>[8x]MAQILPIRFQEHLQLQNLGINPANIGFSTLTMESDKFICIREKVGEQAQVVIIDMNDPSNPIRRPISADSAIMNPASKVIALKAGKTLQIFNIEMKSKMKAHTMTDDVTFWKWISLNTVALVTDNAVYHWSMEGESQPVKMFDRHSSLAGCQIINYRTDAKQKWLLLTGISAQQNRVVGAMQLYSVDRKVSQPIEGHAASFAQFKMEGNAEESTLFCFAVRGQAGGKLHIIEVGTPPTGNQPFPKKAVDVFFPPEAQNDFPVAM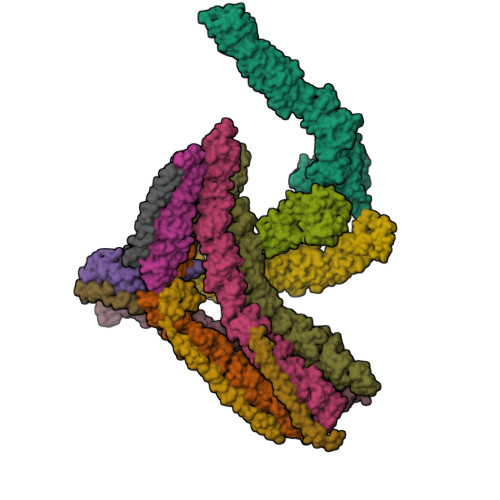QISEKHDVVFLITKYGYIHLYDLETGTCIYMNRISGETIFVTAPHEATAGIIGVNRKGQVLSVCVEEENIIPYITNVLQNPDLALRMAVRNNLAGAEELFARKFNALFAQGNYSEAAKVAANAPKGILRTPDTIRRFQSVPAQPGQTSPLLQYFGILLDQGQLNKYESLELCRPVLQQGRKQLLEKWLKEDKLECSEELGDLVKSVDPTLALSVYLRANVPNKVIQCFAETGQVQKIVLYAKKVGYTPDWIFLLRNVMRISPDQGQQFAQMLVQDEEPLADITQIVDVFMEYNLIQQCTAFLLDALKNNRPSEGPLQTRLLEMNLMHAPQVADAILGNQMFTHYDRAHIAQLCEKAGLLQRALEHFTDLYDIKRAVVHTHLLNPEWLVNYFGSLSVEDSLECLRAMLSANIRQNLQICVQVASKYHEQLSTQSLIELFESFKSFEGLFYFLGSIVNFSQDPDVHFKYIQAACKTGQIKEVERICRESNCYDPERVKNFLKEAKLTDQLPLIIVCDRFDFVHDLVLYLYRNNLQKYIEIYVQKVNPSRLPVVIGGLLDVDCSEDVIKNLILVVRGQFSTDELVAEVEKRNRLKLLLPWLEARIHEGCEEPATHNALAKIYIDSNNNPERFLRENPYYDSRVVGKYCEKRDPHLACVAYERGQCDLELINVCNENSLFKSLSRYLVRRKDPELWGSVLLESNPYRRPLIDQVVQTALSETQDPEEVSVTVKAFMTADLPNELIELLEKIVLDNSVFSEHRNLQNLLILTAIKADRTRVMEYINRLDNYDAPDIANIAISNELFEEAFAIFRKFDVNTSAVQVLIEHIGNLDRAYEFAERCNEPAVWSQLAKAQLQKGMVKEAIDSYIKADDPSSYMEVVQAANTSGNWEELVKYLQMARKKARESYVETELIFALAKTNRLAELEEFINGPNNAHIQQVGDRCYDEKMYDAAKLLYNNVSNFGRLASTLVHLGEYQAAVDGARKANSTRTWKEVCFACVDGKEFRLAQMCGLHIVVHADELEELINYYQDRGYFEELITMLEAALGLERAHMGMFTELAILYSKFKPQKMREHLELFWSRVNIPKVLRAAEQAHLWAELVFLYDKYEEYDNAIITMMNHPTDAWKEGQFKDIITKVANVELYYRAIQFYLEFKPLLLNDLLMVLSPRLDHTRAVNYFSKVKQLPLVKPYLRSVQNHNNKSVNESLNNLFITEEDYQALRTSIDAYDNFDNISLAQRLEKHELIEFRRIAAYLFKGNNRWKQSVELCKKDSLYKDAMQYASESKDTELAEELLQWFLQEEKRECFGACLFTCYDLLRPDVVLETAWRHNIMDFAMPYFIQVMKEYLTKVDKLDASESLRKEEEQATETQ;> MAQILPIRFQEHLQLQNLGINPANIGFSTLTMESDKFICIREKVGEQAQVVIIDMNDPSNPIRRPISADSAIMNPASKVIALKAGKTLQIFNIEMKSKMKAHTMTDDVTFWKWISLNTVALVTDNAVYHWSMEGESQPVKMFDRHSSLAGCQIINYRTDAKQKWLLLTGISAQQNRVVGAMQLYSVDRKVSQPIEGHAASFAQFKMEGNAEESTLFCFAVRGQAGGKLHIIEVGTPPTGNQPFPKKAVDVFFPPEAQNDFPVAMQISEKHDVVFLITKYGYIHLYDLETGTCIYMNRISGETIFVTAPHEATAGIIGVNRKGQVLSVCVEEENIIPYITNVLQNPDLALRMAVRNNLAGAEELFARKFNALFAQGNYSEAAKVAANAPKGILRTPDTIRRFQSVPAQPGQTSPLLQYFGILLDQGQLNKYESLELCRPVLQQGRKQLLEKWLKEDKLECSEELGDLVKSVDPTLALSVYLRANVPNKVIQCFAETGQVQKIVLYAKKVGYTPDWIFLLRNVMRISPDQGQQFAQMLVQDEEPLADITQIVDVFMEYNLIQQCTAFLLDALKNNRPSEGPLQTRLLEMNLMHAPQVADAILGNQMFTHYDRAHIAQLCEKAGLLQRALEHFTDLYDIKRAVVHTHLLNPEWLVNYFGSLSVEDSLECLRAMLSANIRQNLQICVQVASKYHEQLSTQSLIELFESFKSFEGLFYFLGSIVNFSQDPDVHFKYIQAACKTGQIKEVERICRESNCYDPERVKNFLKEAKLTDQLPLIIVCDRFDFVHDLVLYLYRNNLQKYIEIYVQKVNPSRLPVVIGGLLDVDCSEDVIKNLILVVRGQFSTDELVAEVEKRNRLKLLLPWLEARIHEGCTEPATHNALAKIYIDSNNNPERFLRENPYYDSRVVGKYCEKRDPHLACVAYERGQCDLELINVCNENSLFKSLSRYLVRRKDPELWGSVLLESNPYRRPLIDQVVQTALSETQDPEEVSVTVKAFMTADLPNELIELLEKIVLDNSVFSEHRNLQNLLILTAIKADRTRVMEYINRLDNYDAPDIANIAISNELFEEAFAIFRKFDVNTSAVQVLIEHIGNLDRAYEFAERCNEPAVWSQLAKAQLQKGMVKEAIDSYIKADDPSSYMEVVQAANTSGNWEELVKYLQMARKKARESYVETELIFALAKTNRLAELEEFINGPNNAHIQQVGDRCYDEKMYDAAKLLYNNVSNFGRLASTLVHLGEYQAAVDGARKANSTRTWKEVCFACVDGKEFRLAQMCGLHIVVHADELEELINYYQDRGYFEELITMLEAALGLERAHMGMFTELAILYSKFKPQKMREHLELFWSRVNIPKVLRAAEQAHLWAELVFLYDKYEEYDNAIITMMNHPTDAWKEGQFKDIITKVANVELYYRAIQFYLEFKPLLLNDLLMVLSPRLDHTRAVNYFSKVKQLPLVKPYLRSVQNHNNKSVNESLNNLFITEEDYQALRTSIDAYDNFDNISLAQRLEKHELIEFRRIAAYLFKGNNRWKQSVELCKKDSLYKDAMQYASESKDTELAEELLQWFLQEEKRECFGACLFTCYDLLRPDVVLETAWRHNIMDFAMPYFIQVMKEYLTKVDKLDASESLRKEEEQATETQ;>[4x]MADDFGFFSSSESGAPEVAEEDPAAAFLAQQESEIAGIENDEGFGAPAGSQAALAQPGPASGAGPEDMGTTVNGDVFQDANGPADGYAAIAQADRLTQEPESIRKWREEQRKRLQELDAASKVTEQEWREKAKKDLEEWNQRQSEQVEKNKINNRIADKAFYQQPDADIIGYVASEEAFVKESKEETPGTEWEKVAQLCDFNPKSSKQCKDVSRLRSVLMSLKQTPLSR;> GGYVAPKAVWLPAVKAKGLEISGTFTHRQGHIYMEMNFTNKALQHMTDFAIQFNKNSFGVIPSTPLAIHTPLMPNQSIDVSLPLNTLGPVMKMEPLNNLQVAVKNNIDVFYFSCLIPLNVLFVEDGKMERQVFLATWKDIPNENELQFQIKECHLNADTVSSKLQNNNVYTIAKRNVEGQDMLYQSLKLTNGIWILAELRIQPGNPNYTLSLKCRAPEVSQYIYQVYDSILKN>[8x]HHHHHHGSMGYPVIVEATRSPIGKRNGWLSGLHATELLGAVQKAVVDKAGIQSGLHAGDVEQVIGGCVTQFGEQSNNISRVAWLTAGLPEHVGATTVDCQSGSGQQANHLIAGLIAAGAIDVGIACGIEAMS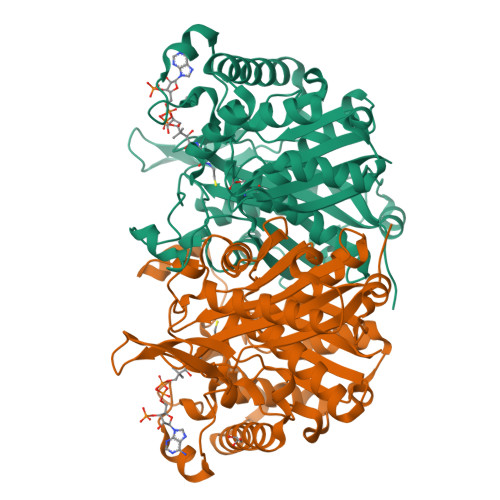RVGLGANAGPDRSLIRAQSWDIDLPNQFEAAERIAKRRGITREDVDVFGLESQRRAQRAWAEGRFDREISPIQAPVLDEQNQPTGERRLVFRDQGLRETTMAGLGELKPVLEGGIHTAGTSSQISDGAAAVLWMDEAVARAHGLTPRARIVAQALVGAEPYYHLDGPVQSTAKVLEKAGMKIGDIDIVEINEAFASVVLSWARVHEPDMDRVNVNGGAIALGHPVGCTGSRLITTALHELERTDQSLALITMCAGGALSTGTIIERI> MHHHHHHHHHHGENLYFQGSDNIISFDHVTFTYPDSPRPALSDLSFAIERGSWTALIGHNGSGKSTVSKLINGLLAPDDLDKSSITVDGVKLGADTVWEVREKVGIVFQNPDNQFVGATVSDDVAFGLENRAVPRPEMLKIVAQAVADVGMADYADSEPSNLSGGQKQRVAIAGILAVKPQVIILDESTSMLDPEGKEQILDLVRKIKEDNNLTVISITHDLEEAAGADQVLVLDDGQLLDQGKPEEIFPKVEMLKRIGLDIPFVYRLKQLLKERGIVLPDEIDDDEKLVQSLW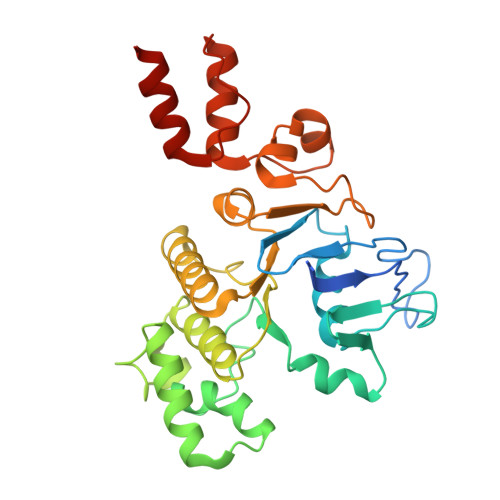QLNSKM> EKVFEEPEEFLKHSQADHLLDEKGKAQSLLQREVVQSLEQQLELEKEKLGAMQAHLAGKMALAKAP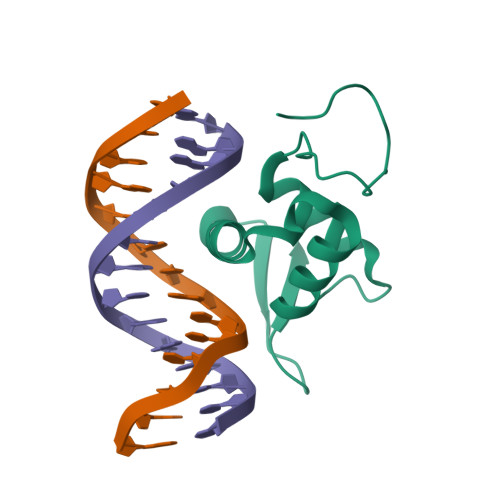SVASMDKPEFFHNMDYFKYHNMRPPFTYATLIRWAILEAPERQRTLNEIYHWFTRMFAYFRNHPATWKNAIRHNLSLHKCFVRVESEKGAVWTVDEFEFRKKR N-[4-[(6-chloranylpyridazin-3-yl)amino]phenyl]-3-(trifluoromethyl)benzamide 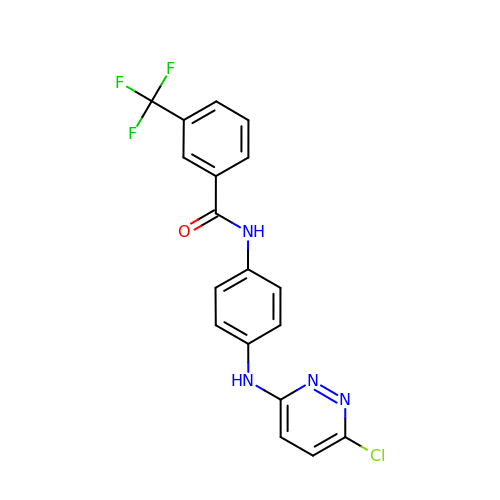| C18 H12 Cl F3 N4 O | JJDWUVWXLMWVFS-UHFFFAOYSA-N> 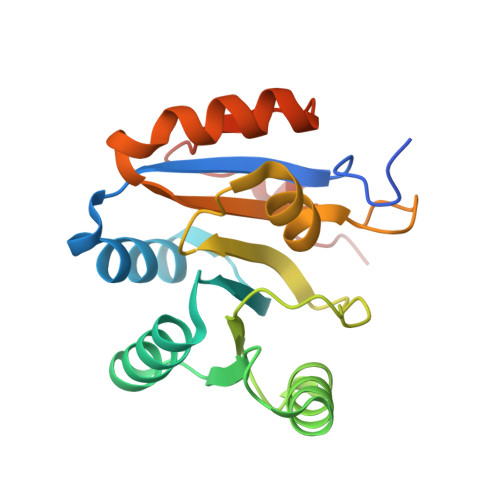MGHHHHHHMEELTLLGVTQYYAFVQEKQKVHCLNTLFRKLQINQSIIFCNSTQRVELLAKKITEIGYSCYYIHSKMAQNHRNRVFHDFRQGNCRNLVCSDLLTRGIDIQAVNVVINFDFPRNAETYLHRIGRSGRFGHLGVAINLITYEDRHTLRRIEQELRTRIEPIPKTVDPKLYVADQQ>TENKILI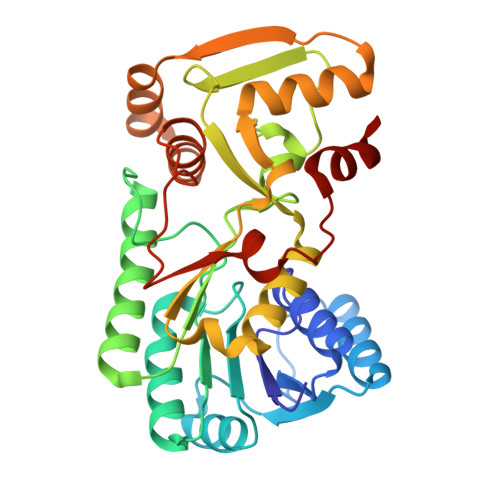LGPTGAIGRHIVWASIKAGNPTYALVRKTITAANPETKEELIDNYQSLGVILLEGDINDHETLVKAIKQVDIVICAAGRLLIEDQVKIIKAIKEAGNVKKFFPSEFGLDVDRHDAVEPVRQVFEEKASIRRVIEAEGVPYTYLCCHAFTGYFLRNLAQLDATDPPRDKVVILGDGNVKGAYVTEADVGTFTIRAANDPNTLNKAVHIRLPKNYLTQNEVIALWEKKIGKTLEKTYVSEEQVLKDIQESSFPHNYLLALYHSQQIKGDAVYEIDPAKDIEASEAYPDVTYTTADEYLNQFV[2x]>DNWRYAHEEYEGDVQDVFAQAFKGYVEDNSDHTVQVYRFGELGESDDIMEQTQNGILQFVNQSPGFTGSLIPSAQIFFIPYLMPTDMDTVLEFFDESKAINEMFPKLYAEHGLELLKMYPEGEMVV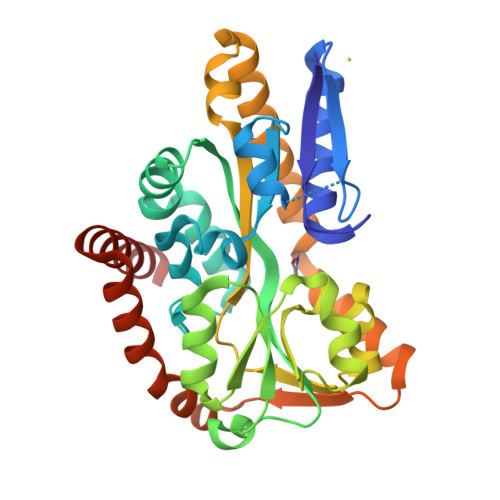TADEPITSPEDFDNKKIRTMTNPLLAETYKAFGATPTPLPWGEVYGGLQTGIIDGQENPIFWIESGGLYEVSPNLTFTSHGWFTTAMMANQDFYEGLSEEDQQLVQDAADAAYDHTIEHIKGLSEESLEKIKAASDEVTVTRLNDEQIQAFKERAPQVEEKFIEMTGEQGQELLDQFKADLKAVQSESEG[2x]> ADTKEVLEAREAYFKSLGGSMKAMTGVAKAFDAEAAKVEAAKLEKILATDVAPLFPAGTSSTDLPGQTEAKAAIWANM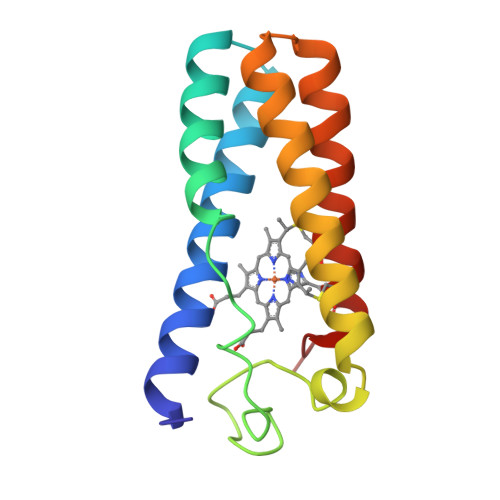DDFGAKGKAMHEAGGAVIAAANAGDGAAFGAALQKLGGTCKACHDDYREED(4-chloranyl-2-methyl-pyrazol-3-yl)-piperidin-1-yl-methanone | C10 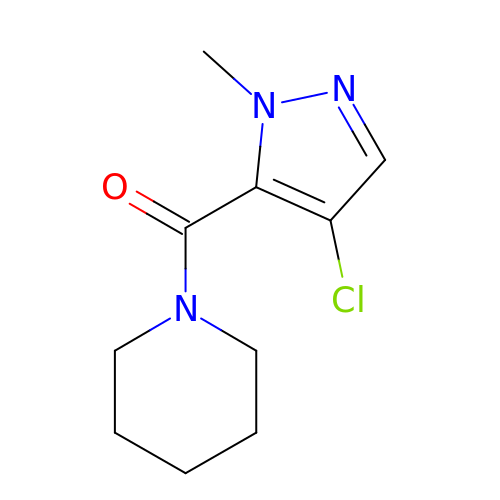H14 Cl N3 O | KRGQOKCRZMRVRH-UHFFFAOYSA-N> TQVLNGYWGYQEFLDEFPEQRNLTNALSEAVRAQPVPLSKPTQRPIKISVVYPGQQVSDYWVRNIASFEKRLYKLNINYQLNQVFTRPNADIKQQSLSLMEALKSKSDYLIFTLDT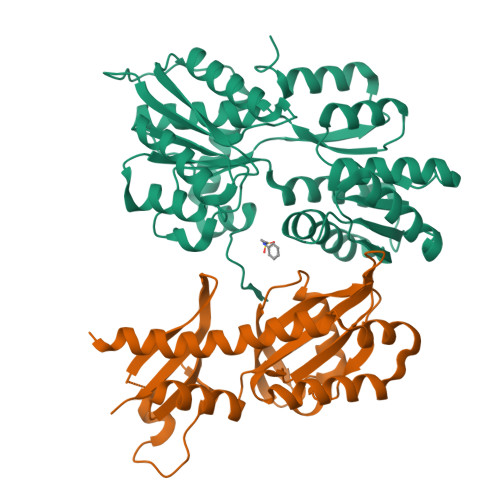TRHRKFVEHVLDSTNTKLILQNITTPVREWDKHQPFLYVGFDHAEGSRELATEFGKFFPKHTYYSVLYFSEGYISDVRGDTFIHQVNRDNNFELQSAYYTKATKQSGYDAAKASLAKHPDVDFIYACSTDVALGAVDALAELGREDIMINGWGGGSAELDAIQKGDLDITVMRMNDDTGIAMAEAIKWDLEDKPVPTVYSGDFEIVTKADSPERIEALKKRAFRYSDN;> GSYFSKQIIWQEVDRTKQQTSALIHNIFDSHFAAIQIHHDSNSKSEVIRDFYTDRDTDVLNFFFLSIDQSDPSHTPEFRFLTDHKGIIWDDGNAHFYGVNDLILDSLANRVSFSNNWYYINVMTSIGSRHMLVRRVPILDPSTGEVLGFSFNAVVLDNNFALMEKLKSESNVDNVVLVANSVPLANSLIGDEPYNVADVLQRKSSDKRLDKLLVIETPIVVNAVTTELCLLTVQDNQSVVTL> GSPPAQLSVHTVSWNSGHERAPTNLEELLGLNSGETPDVIA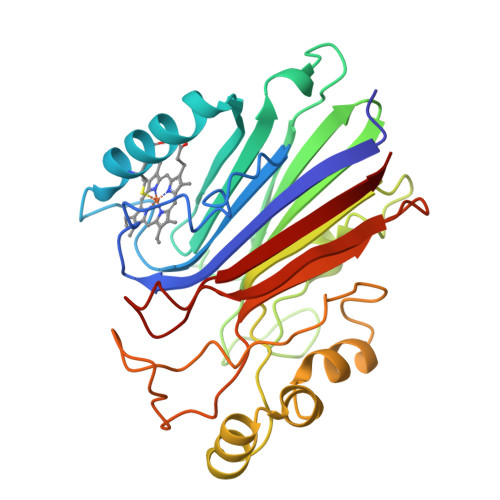VAVQGFGFQTDKPQQGPACVKNFQSLLTSKGYTKLKNTITETMGLTVYCLEKHLDQNTLKNETIIVTVDDQKKSGGIVTSFTIYNKRFSFTTSRMSDEDVTSTNTKYAYDTRLDYSKKDDPSDFLFWIGDLNVRVETNATHAKSLVDQNNIDGLMAFDQLKKAKEQKLFDGWTEPQVTFKPTYKFKPNTDEYDLSATPSWTDRALYKSGTGKTIQPLSYNSLTNYKQTEHRPVLAKFRVTL(4E)-4-AMINOHEX-4-ENOIC ACID | C6 H11 N O2 | 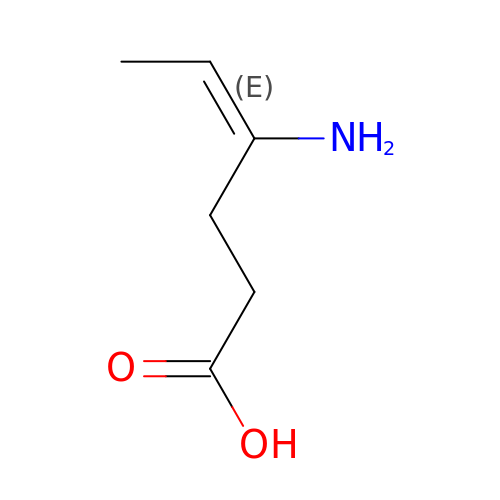KQFBUAIXCIGKAP-GORDUTHDSA-N> TLLTFFATDARLDPAEQDRLFRRVMDRTFNAVSIDTDTSTSDTAVLFANGLAG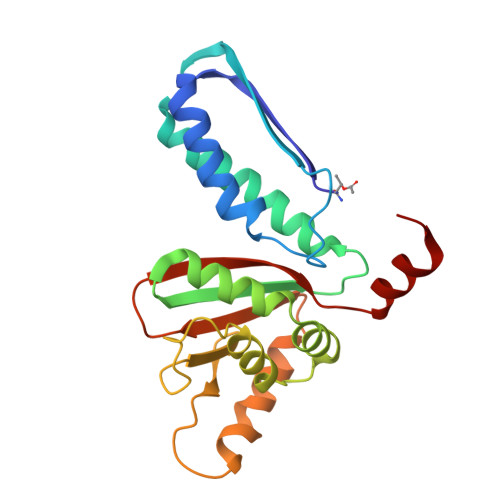EVDAGEFEEALHTAALALVKDIASDGEGAAKLIEVQVTGARDDAQAKRVGKTVVNSPLVKTAVHGCDPNWGRVAMAIGKCSDDTDIDQERVTIRFGEVEVYPPKARGDQADDALRAAVAEHLRGDEVVIGIDLAIADGAFTVYGCDLTEGYVRLNSEYTT> VEMVDNLRGKSGQGYYVEMTVGSPPQTLNILVDTGSSNFAVGAAPHPFLHRYYQRQLSSTYRDLRKGVYVPYTQGKWEGELGTDLVSIPHGPNVTVRANIAAITESDKFFINGSNWEGILGLAYAEIARPDDSLEPFFDSLVKQTHVPNLFSLQLCGAGFPLNQSEVLASVGGSMIIGGIDHSLYTGSLWYTPIRREWYYEVIIVRVEINGQDLKMDCKEYNYDKSIVDSGTTNLRLPKKVFEAAVKSIKAASSTEKFPDGFWLGEQLVCWQAGTTPWNIFPVISLYLMGEVTNQSFRITILPQQYLRPVEDVATSQDDCYKFAISQSSTGTVMGAVIMEGFYVVFDRA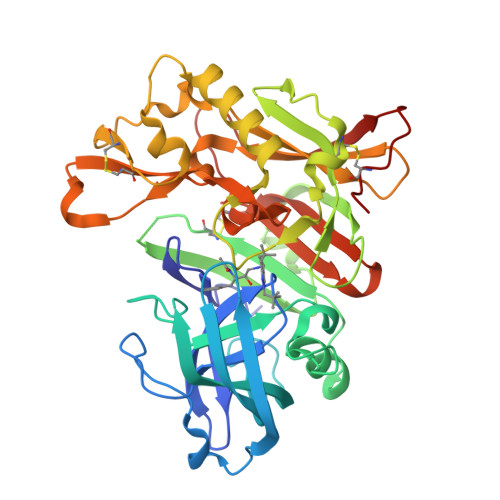RKRIGFAVSACHVHDEFRTAAVEGPFVTLDMEDCGYN>QEG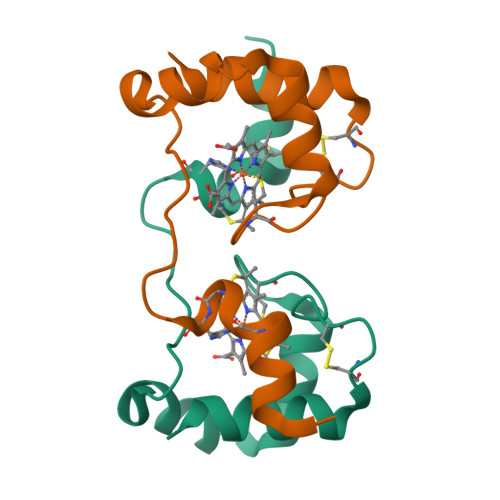KAVYDKACHICHSMGVAGAPKAHDAAAWEPRIAQGLDTLVSTVKTGKGAMPPGGMCTDCTDEDYKSAIEYMSK[2x]ACBD3 is a Golgi resident protein involved in the maintenance of the Golgi structure and regulation of intracellular trafficking between the endoplasmic reticulum and the Golgi. However, in enterovirus-infected cells, the ACBD3 GOLD domain interacts preferentially with viral non-structural 3A proteins, which causes re-localization of ACBD3 to the sites of virus replication. In this study, we present a structural, biochemical, and biological characterization of the complexes composed of human ACBD3 and the 3A proteins of four representative enteroviruses. The crystal structures revealed the details of the ACBD3-3A interaction, the 3A-3A interaction causing the assembly of the ACBD3-3A heterotetramers, the interaction between the ACBD3-3A complex and the lipid bilayer, and the roles of these interactions in facilitation of enterovirus replication.

Of the six GOLD: enterovirus 3A complexes, only GOLD: 3A/EVD68 and GOLD: 3A/RVB14 formed crystals that diffracted to a resolution suitable for subsequent structure determination (i.e. 2.3 Å and 2.9 Å, respectively). For this analysis, we chose the GOLD: EVD68 3A complex because we resolved its structure at the highest resolution. In the GOLD: EVD68 3A crystal structure, we could trace the polypeptide chain of the 3A protein from T163A to I583A. It contains four secondary elements: two alpha helices P193A-V293A (α13A) and Q323A-K413A (α23A), and two beta strands I443A-I463A (β13A) and V533A-I583A (β23A). All these segments contribute to the GOLD: 3A interaction mediated through multiple hydrophobic interactions and hydrogen bonds. The helices α13A and α23A bind to a mild cavity of the GOLD domain that is formed by four antiparallel beta strands of ACBD3. The strand β13A interacts with the strand K518ACBD3-R528ACBD3 of the ACBD3 GOLD domain, while the strand β23A binds to the strand V402ACBD3-P408ACBD3, both in the antiparallel orientation. The dimerization interface of the GOLD: 3A/EVD68 complex consists of the hydrophobic core formed by the residues L25, V29, V34, and Y37, and an additional intermolecular salt bridge between the residues D24 and K41. Analysis of the crystal structures of the GOLD: 3A complexes revealed that the 3A proteins formed either one of the crystal-packing contacts (as in the case of EVD68 and PV1) or contacts with the second 3A molecule when two GOLD: 3A complexes per asymmetric unit were present (as in the case of EVA71 and RVB14). The dissociation constants of the GOLD: enterovirus 3A complexes ranged approximately from 1 μM (EVD68 and RVB14) to 15 μM (EVA71).

> MESLPVIAAPSMWTRPQIKDFKEKIQQDADSVITVGRGEVVTVRVPTHEEGSYLFWEFATDNYDIGFGVYFEWTDSPNTAVSVHVSESSDDDEEEEENIGCEEKAKKNANKPLLDEIVPVYRRDCHEEVYAGSHQYPGRGVYLLKFDNSYSLWRSKSVYYRVYYTR;> GAMGPPQFKEIKISVAPDTPAPDAINDLLRSVDSQEVRDYCQKKGWIVIHPSNELVVEKHISR3-(dimethylamino)butyl dimethylcarbamate | C9 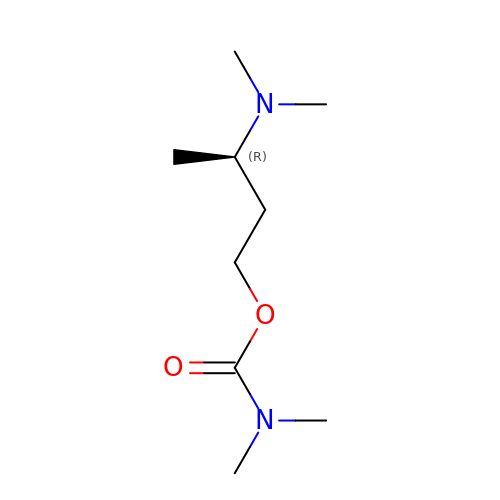H20 N2 O2 | VVGQXMCHKFOTKZ-MRVPVSSYSA-N> MAFHVEGLIAIIVFYLLILLVGIWAAWRTKNSGSAEERSEAIIVGGRDIGLLVGGFTMTATWVGGGYINGTAEAVYVPGYGLAWAQAPIGYSLSLILGGLFFAKPMRSKGYVTMLDPFQQIYGKRMGGLLFIPALMGEMFWAAAIFSALGATISVIIDVDMHISVIISALIATLYTLVGGLYSVAYTDVVQLFCIFVGLWISVPFALSHPAVADIGFTAVHAKYQKPWLGTVDSSEVYSWLDSFLLLMLGGIPWQAYFQRVLSSSSATYAQVLSFLAAFGCLVMAIPAILIGAIGASTDWNQTAYGLPDPKTTEEADMILPIVLQYLCPVYISFFGLGAVSAAVMSSADSSILSASSMFARNIYQLSFRQNASDKEIVWVMRITVFVFGASATAMALLTKTVYGLWYLSSDLVYIVI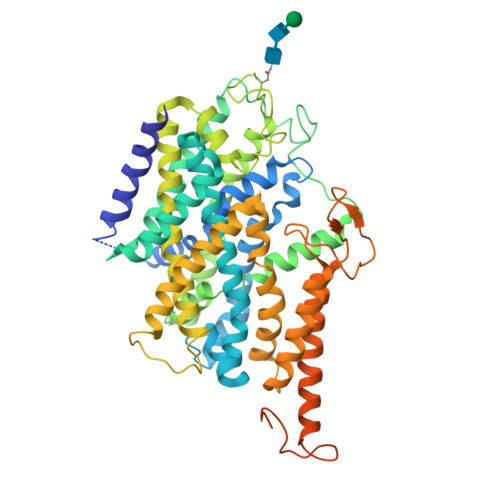FPQLLCVLFVKGTNTYGAVAGYVSGLFLRITGGEPYLYLQPLIFYPGYYPDDNGIYNQKFPFKTLAMVTSFLTNICISYLAKYLFESGTLPPKLDVFDAVVARHSEENMDKTILVKNENIKLDELALVKPRQSMTLSSTFTNKEAFLDVDSSPEGSGTEDNLQ> MRHPLQCHW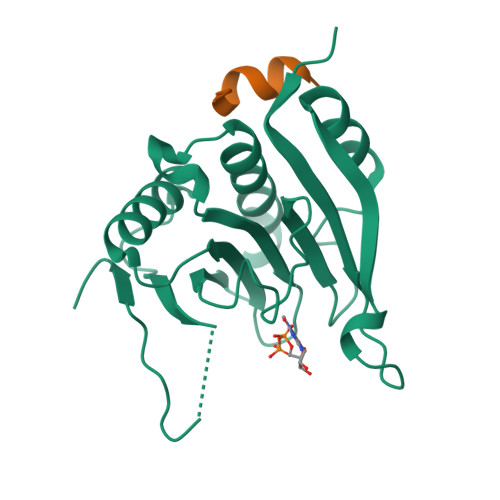ALWYLKADRSKDWEDCLKQVAVFDTVEDFWSLYNHIQAASGLTWGSDYYLFKEGIKPMWEDENNVKGGRWLVVVDKQKRAQLLDHYWLELLMAIIGEQFEDNGEYICGAVVNVRQKGDKVSLWTRDSLKDDVNLRIGQILKAKLEIPDTEPIRYEVHKDSSVRTGSMVKPRIVIPSKDNR;> RIIYDRKFLMECRNSPV> MLTAHHLDVARRHGTILRDLSLSIEPGRVTALLGRNGAGKSTLLKTFAGELTGSVAPHGVRVTGDVTLNGEPLARIDAPRLACLRAVLPQAAQPAFPFSVDEIVLLGR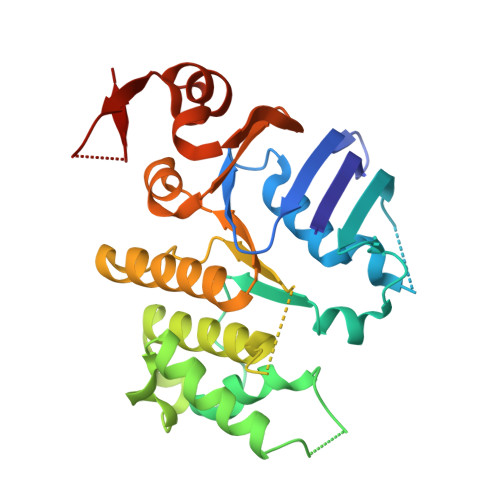YPHARRSGATSHRDRDIAWRALERAGADALVGRDVTTLSGGELARVQFARVLAQLWPDHDTTEPGPRYLLLDEPTAALDLAHQHRLLDTVRAVAREWQLGVLAIVHDPNLAARHADAIAMLADGTIVAHGAPRDVMTPAHIAQCYGFAVKMVETGDGTPPVMVPA>MNESVKEIPDVLKSQCGFNCLTDISHSSFNEFRQQVSEHLSWSETHDLYHDAQQAQKDNRLYEARILKRANPQLQNAVHLAILAPNAELIGYNNQFSGRASQYVAPGTVSSMFSPAAYLTELYREARNLHASDSVYYLDTRRPDLKSMALSQQNMDIELSTLSLSNELLLESIKTESKLENYTKVMEMLSTFRPSGATPYHDAYENVREVIQLQDPGLEQLNASPAIAGLMHQASLLGINASISPELFNILTEEITEGNAEELYKKNFGNIEPASLAMPEYLKRYYNLSDEELSQFIGKASNFGQQEYSNNQLITPVVNSSDGTVKVYRITREYTTNAYQMDVELFPFGGENYRLDYKFKNFYNASYLSIKLNDKRELVRTEGAPQVNIEYSANITLNTADISQPFEIGLTRVLPSGSWAYAAAKFTVEEYNQYSFLLKLNKAIRLSRATELSPTILEGIVRSVNLQLDINTDVLGKVFLTKYYMQRYAIHAETALILCNAPISQRSYDNQPSQFDRLFNTPLLNGQYFSTGDEEIDLNSGSTGDWRKTILKRAFNIDDVSLFRLLKITDHDNKDGKIKNNLKNLSNLYIGKLLADIHQLTIDELDLLLIAVGEGKTNLSAISDKQLATLIRKLNTITSWLHTQKWSVFQLFIMTSTSYNKTLTPEIKNLLDTVYHGLQGFDKDKADLLHVMAPYIAATLQLSSENVAHSVLLWADKLQPGDGAMTAEKFWDWLNTKYTPGSSEAVETQEHIVQYCQALAQLEMVYHSTGINENAFRLFVTKPEMFGAATGAAPAHDALSLIMLTRFADWVNALGEKASSVLAAFEANSLTAEQLADAMNLDANLLLQASIQAQNHQHLPPVTPENAFSCWTSINTILQWVNVAQQLNVAPQGVSALVGLDYIESMKETPTYAQWENAAGVLTAGLNSQQANTLHAFLDESRSAALSTYYIRQVAKAAAAIKSRDDLYQYLLIDNQVSAAIKTTRIAEAIASIQLYVNRALENVEENANSGVISRQFFIDWDKYNKRYSTWAGVSQLVYYPENYIDPTMRIGQTKMMDALLQSVSQSQLNADTVEDAFMSYLTSFEQVANLKVISAYHDNINNDQGLTYFIGLSETDAGEYYWRSVDHSKFNDGKFAANAWSEWHKIDCPINPYKSTIRPVIYKSRLYLLWLEQKEITKQTGNSKDGYQTETDYRYELKLAHIRYDGTWNTPITFDVNKKISELKLEKNRAPGLYCAGYQGEDTLLVMFYNQQDTLDSYKNASMQGLYIFADMASKDMTPEQSNVYRDNSYQQFDTNNVRRVNNRYAEDYEIPSSVSSRKDYGWGDYYLSMVYNGDIPTINYKAASSDLKIYISPKLRIIHNGYEGQKRNQCNLMNKYGKLGDKFIVYTSLGVNPNNSSNKLMFYPVYQYSGNTSGLNQGRLLFHRDTTYPSKVEAWIPGAKRSLTNQNAAIGDDYATDSLNKPDDLKQYIFMTDSKGTATDVSGPVEINTAISPAKVQIIVKAGGKEQTFTADKDVSIQPSPSFDEMNYQFNALEIDGSGLNFINNSASIDVTFTAFAEDGRKLGYESFSIPVTLKVSTDNALTLHHNENGAQYMQWQSYRTRLNTLFARQLVARATTGIDTILSMETQNIQEPQLGKGFYATFVIPPYNLSTHGDERWFKLYIKHVVDNNSHIIYSGQLTDTNINITLFIPLDDVPLNQDYHAKVYMTFKKSPSDGTWWGPHFVRDDKGIVTINPKSILTHFESVNVLNNISSEPMDFSGANSLYFWELFYYTPMLVAQRLLHEQNFDEANRWLKYVWSPSGYIVHGQIQNYQWNVRPLLEDTSWNSDPLDSVDPDAVAQHDPMHYKVSTFMRTLDLLIARGDHAYRQLERDTLNEAKMWYMQALHLLGDKPYLPLSTTWSDPRLDRAADITTQNAHDSAIVALRQNIPTPAPLSLRSANTLTDLFLPQINEVMMNYWQTLAQRVYNLRHNLSIDGQPLYLPIYATPADPKALLSAAVATSQGGGKLPESFMSLWRFPHMLENARGMVSQLTQFGSTLQNIIERQDAEALNALLQNQAAELILTNLSIQDKTIEELDAEKTVLEKSKAGAQSRFDSYGKLYDENINAGENQAMTLRASAAGLTTAVQASRLAGAAADLVPNIFGFAGGGSRWGAIAEATGYVMEFSANVMNTEADKISQSETYRRRRQEWEIQRNNAEAELKQIDAQLKSLAVRREAAVLQKTSLKTQQEQTQSQLAFLQRKFSNQALYNWLRGRLAAIYFQFYDLAVARCLMAEQAYRWELNDDSARFIKPGAWQGTYAGLLAGETLMLSLAQMEDAHLKRDKRALEVERTVSLAEVYAGLPKDNGPFSLAQEIDKLVSQGSGSAGSGNNNLAFGAGTDTKTSLQASVSFADLKIREDYPASLGKIRRIKQISVTLPALLGPYQDVQAILSYGDKAGLANGCEALAVSHGMNDSGQFQLDFNDGKFLPFEGIAIDQGTLTLSFPNASMPEKGKQATMLKTLNDIILHIRYTIK[5x];> MQNSQDFSITELSLPKGGGAITGMGEALTPTGPDGMAALSLPLPISAGRGYAPAFTLNYNSGAGNSPFGLGWDCNVMTIRRRTHFGVPHYDETDTFLGPEGEVLVVADQPRDESTLQGINLGATFTVTGYRSRLESHFSRLEYWQPKTTGKTDFWLIYSPDGQVHLLGKSPQARISNPSQTTQTAQWLLEASVSSRGEQIYYQYRAEDDTGCEADEITHHLQATAQRYLHIVYYGNRTASETLPGLDGSAPSQADWLFYLVFDYGERSNNLKTPPAFSTTGSWLCRQDRFSRYEYGFEIRTRRLCRQVLMYHHLQALDSKITEHNGPTLVSRLILNYDESAIASTLVFVRRVGHEQDGNVVTLPPLELAYQDFSPRHHAHWQPMDVLANFNAIQRWQLVDLKGEGLPGLLYQDKGAWWYRSAQRLGEIGSDAVTWEKMQPLSVIPSLQSNASLVDINGDGQLDWVITGPGLRGYHSQRPDGSWTRFTPLNALPVEYTHPRAQLADLMGAGLSDLVLIGPKSVRLYANTRDGFAKGKDVVQSGEITLPVPGADPRKLVAFSDVLGSGQAHLVEVSATKVTCWPNLGRGRFGQPITLPGFSQPATEFNPAQVYLADLDGSGPTDLIYVHTNRLDIFLNKSGNGFAEPVTLRFPEGLRFDHTCQLQMADVQGLGVASLILSVPHMSPHHWRCDLTNMKPWLLNEMNNNMGVHHTLRYRSSSQFWLDEKAAALTTGQTPVCYLPFPIHTLWQTETEDEISGNKLVTTLRYARGAWDGREREFRGFGYVEQTDSHQLAQGNAPERTPPALTKNWYATGLPVIDNALSTEYWRDDQAFAGFSPRFTTWQDNKDVPLTPEDDNSRYWFNRALKGQLLRSELYGLDDSTNKHVPYTVTEFRSQVRRLQHTDSRYPVLWSSVVESRNYHYERIASDPQCSQNITLSSDRFGQPLKQLSVQYPRRQQPAINLYPDTLPDKLLANSYDDQQRQLRLTYQQSSWHHLTNNTVRVLGLPDSTRSDIFTYGAENVPAGGLNLELLSDKNSLIADDKPREYLGQQKTAYTDGQNTTPLQTPTRQALIAFTETTVFNQSTLSAFNGSIPSDKLSTTLEQAGYQQTNYLFPRTGEDKVWVAHHGYTDYGTAAQFWRPQKQSNTQLTGKITLIWDANYCVVVQTRDAAGLTTSAKYDWRFLTPVQLTDINDNQHLITLDALGRPITLRFWGTENGKMTGYSSPEKASFSPPSDVNAAIELKKPLPVAQCQVYAPESWMPVLSQKTFNRLAEQDWQKLYNARIITEDGRICTLAYRRWVQSQKAIPQLISLLNNGPRLPPHSLTLTTDRYDHDPEQQIRQQVVFSDGFGRLLQAAARHEAGMARQRNEDGSLIINVQHTENRWAVTGRTEYDNKGQPIRTYQPYFLNDWRYVSNDSARQEKEAYADTHVYDPIGREIKVITAKGWFRRTLFTPWFTVNEDENDTAAEVKKVKMPGSRPMKNIDPKLYQKTPTVSVYDNRGLIIRNIDFHRTTANGDPDTRITRHQYDIHGHLNQSIDPRLYEAKQTNNTIKPNFLWQYDLTGNPLCTESIDAGRTVTLNDIEGRPLLTVTATGVIQTRQYETSSLPGRLLSVAEQTPEEKTSRITERLIWAGNTEAEKDHNLAGQCVRHYDTAGVTRLESLSLTGTVLSQSSQLLIDTQEANWTGDNETVWQNMLADDIYTTLSTFDATGALLTQTDAKGNIQRLAYDVAGQLNGSWLTLKGQTEQVIIKSLTYSAAGQKLREEHGNDVITEYSYEPETQRLIGIKTRRPSDTKVLQDLRYEYDPVGNVISIRNDAEATRFWHNQKVMPENTYTYDSLYQLISATGREMANIGQQSHQFPSPALPSDNNTYTNYTRTYTYDRGGNLTKIQHSSPATQNNYTTNITVSNRSNRAVLSTLTEDPAQVDALF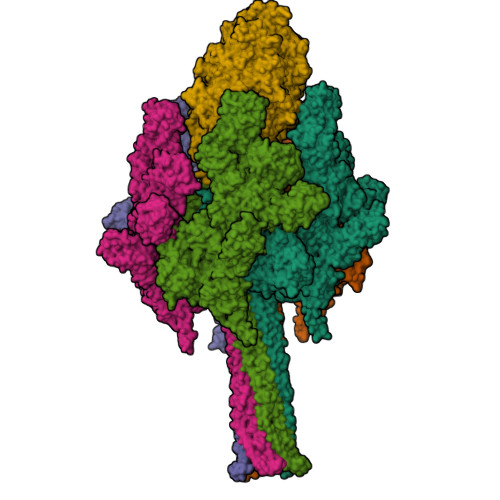DAGGHQNTLISGQNLNWNTRGELQQVTLVKRDKGANDDREWYRYSGDGRRMLKINEQQASNNAQTQRVTYLPNLELRLTQNSTATTEDLQVITVGEAGRAQVRVLHWESGKPEDIDNNQLRYSYDNLIGSSQLELDSEGQIISEEEYYPYGGTALWAARNQTEASYKTIRYSGKERDATGLYYYGYRYYQPWIGRWLSSAPAGTIDGLNLYRMVRNNPVTLLDPDGLMPTIAERIAALKKNKVTDSAPSPANATNVAINIRPPVAPKPSLPKASTSSQPTTHPIGAANIKPTTSGSSIVAPLSPVGNKSTSEISLPESAQSSSSSTTSTNLQKKSFTLYRADNRSFEEMQSKFPEGFKAWTPLDTKMARQFASIFIGQKDTSNLPKETVKNISTWGAKPKLKDLSNYIKYTKDKSTVWVSTAINTEAGGQSSGAPLHKIDMDLYEFAIDGQKLNPLPEGRTKNMVPSLLLDTPQIETSSIIALNHGPVNDAEISFLTTIPLKNVKPHKR> LPRETDEEPEEPGRRGSFVEMVDNLRGKSGQGYYVEMTVGSPPQTLNILVDTGSSNFAVGAAPHPFLHRYYQRQLSSTYRDLRKGVYVPYTQGKWEGELGTDLVSIPHGPNVTVRANIAAITESDKFFINGSNWEGILGLAYAEIARPDDSLEPFFDSLVKQTHVPNLFSLQLCGAGFPLNQSEVLASVGGSMIIGGIDHSLYTGSLWYTPIRREWYYEVIIVRVEINGQDLKMDCKEYNYDKSIVDSGTTNLRLPKKVFEAAVKSIKAASSTEKFPDGFWLGEQLVCWQAGTTPWNIFPVISLY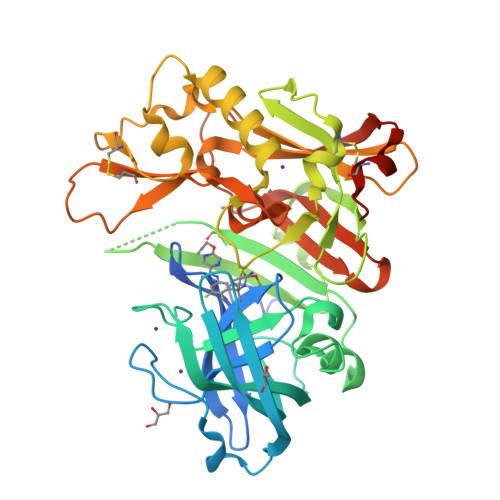LMGEVTNQSFRITILPQQYLRPVEDVATSQDDCYKFAISQSSTGTVMGAVIMEGFYVVFDRARKRIGFAVSACHVHDEFRTAAVEGPFVTLDMEDCGYNIPQTDES>[2x]VANTTYKAPIERPEDFLKDKEKAKEWERKEAERIEQKLERSEKEALESYKKDSVEISKYSQTRNYFYDYQIEANSREKEYKELRNA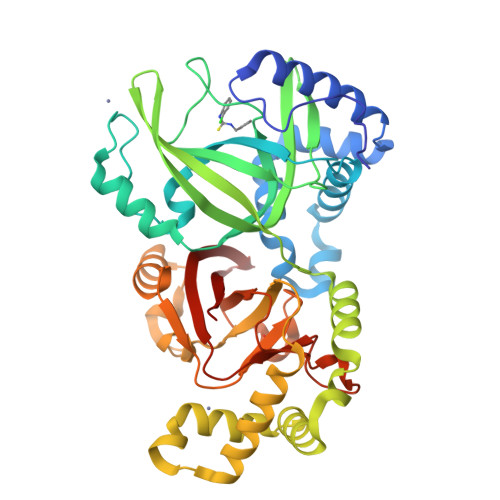ISKNKIDKPMYVYYFESPEKFAFNKVIRTENQNEISLEKFNEFKETIQNKLFKQDGFKDISLYEPGKGDEKPTPLLMHLKLPRNTGMLPYTNTNNVSTLIEQGYSIKIDKIVRIVIDGKHYIKAEASVVSSLDFKDDVSKGDSWGKANYNDWSNKLTPNELADVNDYMRGGYTAINNYLISNGPVNNPNPELDSKITNIENALKREPIPTNLTVYRRSGPQEFGLTLTSPEYDFNKLENIDAFKSKWEGQALSYPNFISTSIGSVNMSAFAKRKIVLRITIPKGSPGAYLSAIPGYAGEYEVLLNHGSKFKINKIDSYKDGTITKLIVDATLIP>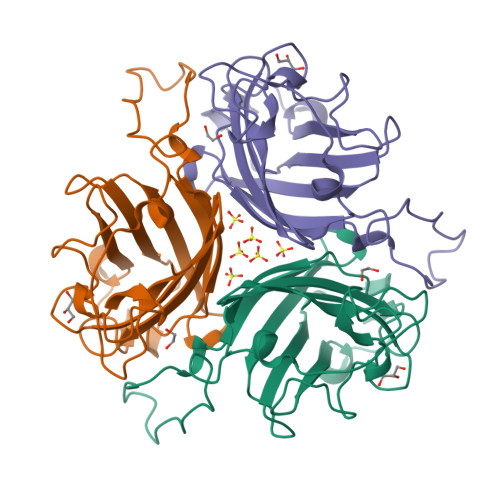[2x]DKLTLWTTPDPSPNCKIDQDKDSKLTFVLTKCGSQILANMSLLVVKGKFSMINNKVNGTDDYKKFTIKLLFDEKGVLLKDSSLDKEYWNYRSNNNNVGSAYEEAVGFMPSTTAYPKPPTPPTNPTTPLEKSQAKNKYVSNVYLGGQAGNPVATTVSFNKETGCTYSITFDFAWNKTYENVQFDSSFLTFSYIAQE>TSAPVPPLIKEATYIEATASGYMAEGVLNPTIILRRGQRVDMTLKNKLTEPTIVHWHGFDVNWHNDAHPSFAITPGESYNYSFDVVNRAGTYLYHPHPHGLTAKQFYMGQLGLVIVEDSGSDLGFKYGVNDLPLVISDRRFIGGAPVYNPTPMEMIAGFLGNAVLVNGIKDAVFKLSGGSYRLRLVNGSNARLYMLSIVKKNGDVVPMRLIAVDQGFLARPIEVRALFLAPAERAEVVVELGEGVYLLKNTPFDHMHLEMGHGMQEALPEGSEYTIATFLVEGKGEAVPVEALPDPPPEPPKPTRTRRFALSLSGMQWTINGMSWNASNPLFEHVSVEGVELWEIVNDKASMTHPVHLHGFPMWIIERKDSPRQVAELAVDNRGRLPTDLGLKDTVLIWPGETVKIVVNFDAKKRGQLFPFHCHNLEHEDGGMMINIAVK[2x]

Multicopper oxidases (MCOs) are proteins composed of three Greek key β-barrel cupredoxin domains (domains 1, 2, and 3) that come together to form three spectroscopically different Cu sites: type 1 (T1), type 2 (T2) and the binuclear type 3 (T3). MCOs couple the one-electron oxidation of substrates at the T1CU with the four-electron reduction of molecular oxygen to water at the T2/T3 trinuclear copper (TNC). The substrates of MCOs vary from organic compounds to metal ions such as Fe(II), Mn(II), and Cu(I) and the family is generally divided into two classes, metalloxidases and laccases. In this study, we engineered the hyperthermophilic metallo-oxidase Pyrobaculum aerophilum McoP to enhance its activity for aromatics, resembling laccase activity, using directed evolution (DE).

The hit variant 1B5 of the fifth generation contained 12 mutations; to reduce to the smallest subset of mutations, the last round of evolution was performed with DNA-shuffling of genes coding for wild-type and 1B5. A library of variants (~ 4200 clones) was screened for ABTS activity, and variant 3F3, with only six mutations, was selected for further studies. The 3F3 variant selected after DNA shuffling showed a ~ tenfold higher kcat than the 1B5 and a remarkable 2-order of magnitude higher kcat/Km compared to wild-type. The analysis of the X-ray crystal structure reveals four proximal mutations close to the T1Cu active site. In McoP, a 23-residue loop 288TPFDHMHLEMGHGMQEALPEGSE310 and a short α-helix (188–195) are occluding the T1Cu. The overall average B-factor value of 3F3 (49 Å2) is higher than the wild-type enzyme (32 Å2), and the loop 288–310 in the 3F3 is the region that shows higher flexibility, with B-factor values ranging from 43–69 Å2 (vs. 22–58 Å2). Part of this loop (segment 296EMGHGMQ302) is not even visible in the electron density maps and was modeled with AlphaFold2 applying a local energy minimization using Yasara. The observed increase in flexibility of the loop in the 3F3 variant may be attributed to structural rearrangements resulting from mutations in the loop, such as P292H, as well as mutations close to the T1CU site, like P390T. The increased flexibility of the loop 288–310 in 3F3 caused structural alterations at the entrance of the tunnel: it is more polar than in the wild-type and has a larger diameter access entry (4.0 Å vs. 2.8 Å) due to the shorter distance between H294 and H292 (3 Å vs. 5 Å). In 3F3, W355, which is located at a distance of 3.4 Å from H465, exhibits significantly greater exposure to the solvent than in the wild-type.The rotating flagellar filament primarily functions as a propeller, acting as an Archimedean screw, and supercoiling of the filament is essential as rotations of a straight filament do not generate thrust. Here, we show the atomic cryo-electron microscopy structures for flagellar filaments from enterohemorrhagic Escherichia coli O157:H7, enteropathogenic E. coli O127:H6, Achromobacter, and Sinorhizobium meliloti, where the outer domains dimerize or tetramerize to form either a sheath or a screw-like surface. A shared feature in all four structures is the formation of symmetrical homodimers between the outer domains of flagellin subunits, with one outer domain rotated 180° relative to the other. These symmetrical dimers are the result of outer domains being able to adopt either an “up” or “down” conformation.

Since a seam breaks the helical symmetry in the EPEC O127:H6 flagellar filament, reconstruction was performed asymmetrically to 4.0 Å. The power spectrum of the EPEC O127:H6 flagellar filament superficially looks similar to the tetrameric Achromobacter filament. However, the Bessel order of many of the layer lines must be different because the EPEC H6 outer domains cannot be reconstructed using the tetrameric flagella symmetry of Achromobacter. We have determined that this is a result of a seam. The EPEC H6 filament ODS is created by an outer domain tetramer with most flagellins being in one of four flagellin outer domain conformations, but the details of this tetramerization are quite different from those in Achromobacter. Due to the presence of the seam, most but not all D2 domains are in one of these four conformations. In one dimer conformation, “D2 Dimer A”, domain D2 of one subunit forms a dimer with D2 from another flagellin that is 11 subunits away. In the other conformation, “D2 Dimer B”, flagellins that are 6-subunits away (Sn:Sn + 6) form dimers with each other. These two dimer conformations are easily observed in the 4.0 Å EPEC H6 map. While a large region of the ODS has very poor density, the resolution of another portion allows the creation of an ab initio atomic model of the complete flagellin structure.

>[23x]QVINTNSLSLITQNNINKNQSALSSSIERLSSGLRINSAKDDAAGQAIANRFTSNIKGLTQAARNANDGISVAQTTEGALSEINNNLQRIRELTVQASTGTNSDSDLDSIQDEIKSRLDEIDRVSGQTQFNGVNVLAKDGSMKIQVGANDGQTITIDLKKIDSDTLGLNGFNVNGKGETANTAATLKDMSGFTAAAAPGGTVGVTQYTDKSAVASSVDILNAVAGADGNKVTTSADVGFGTPAAAVTYTYNKDTNSYSAASDDISSANLAAFLNPQARDTTKATVTIGGKDQDVNIDKSGNLTAADDGAVLYMDATGNLTKNNAGGDTQATLAKVATATGAKAATIQTDKGTFTSDGTAFDGASMSIDANTFANAVKNDTYTATVGAKTYSVTTGSAAADTAYMSNGVLSDTPPTYYAQADGSITTTEDAAAGKLVYKGSDGKLTTDTTSKAESTSDPLAALDDAISQIDKFRSSLGAVQNRLDSAVTNLNNTTTNLSEAQSRIQDADYATEVSNMSKAQIIQQAGNSVLAKANQVPQQVLSLLQG8-IODO-GUANINE 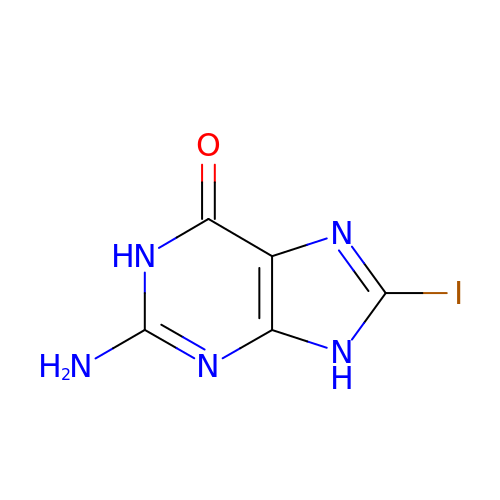| C5 H4 I N5 O | SXGFECRAKVVEJT-UHFFFAOYSA-N>[2x]EDVPQPPVSQFYIQGQVYCDTCRARFITELSEFIPGAGVRLQCKDGENGKIT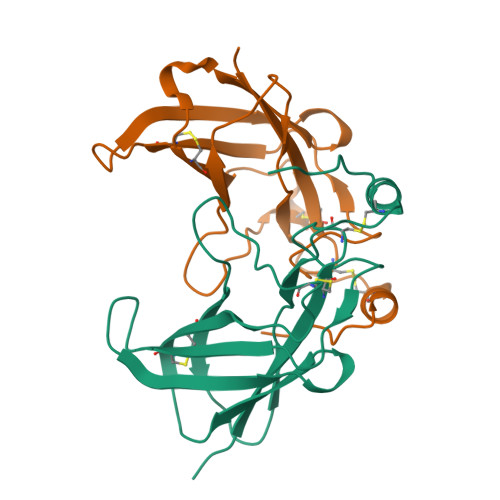FTEVGYTRAEGLYSMLIERDHKNEFCEITLLSSSRKDCDEIPIEGWVKPSLKFMLNTVNGTTRTINPLGFFKKEALPKCPQVFNKLGMYPPNM> 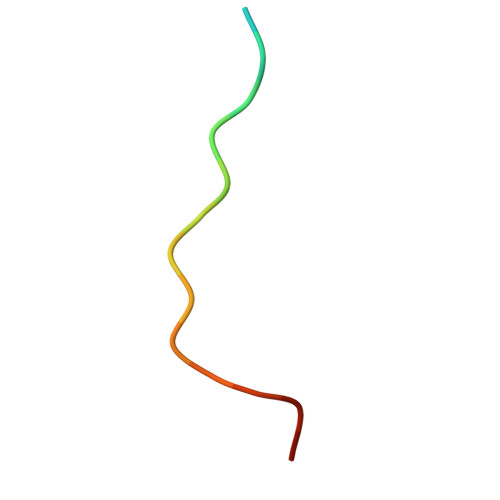TAKQPPVPPPRKKRISX>[4x]MDAVKKAILGEVLEEEEAYEVMRALMAGEVSPVRAAGLLVALSLRGERPHEIAAMARAMREAARPLRVHRRPLLDIVGTGGDGKGLMNLSTLAALVAAAGGVAVAKHGNRAASSRAGSADLLEALGVDLEAPPERVGEAIEELGFGFLFARVFHPAMRHVAPVRAELGVRTVFNLLGPLTNPAGADAYVLGVFSPEWL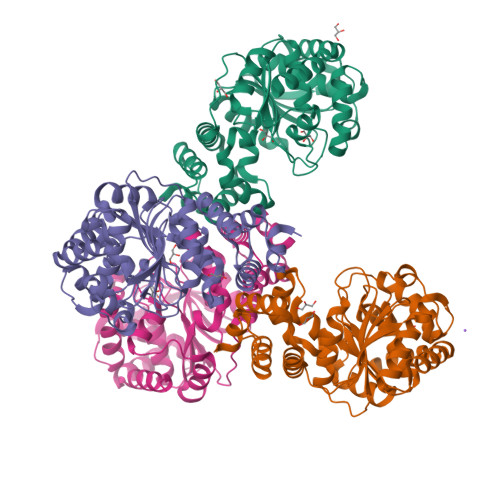APMAEALERLGARGLVVHGEGADELVLGENRVVEVGKGAYALTPEEVGLKRAPLEALKGGGPEENAALARRLLKGEEKGPLADAVALAAGAGFYAAGKTPSLKEGVALAREVLASGEAYLLLERYVAFLRA>[30x]MVLGKVVGTVVASRKEPRIEGLSLLLVRACDPDGTPTGGAVVCADAVGAGVGEVVLYASGSSARQTEVTNNRPVDATIMAIVDLVEMGGDVRFRKD;>[180x]MADALGMIEVRGFVGMVEAA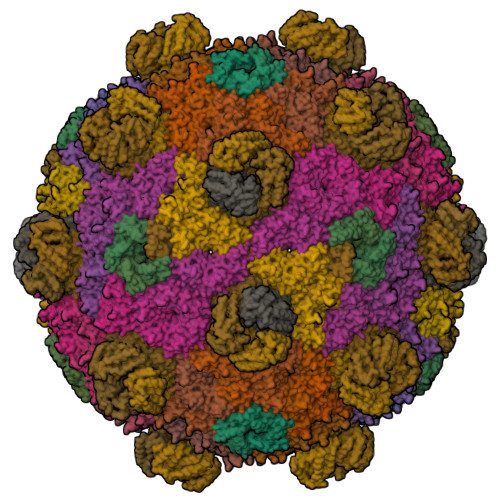DAMVKAAKVELIGYEKTGGGYVTAVVRGDVAAVKAATEAGQRAAERVGEVVAVHVIPRPHVNVDAALPLGRTPGMDKSA;>[60x]MSITLRTYIFLDALQPQLATFIGKTARGFLPVPGQASLWVEIAPGIAINRVTDAALKATKVQPAVQVVERAYGLLEVHHFDQGEVLAAGSTILDKLEVREEGRLKPQVMTHQIIRAVEAYQTQIINRNSQGMMILPGESLFILETQPAGYAVLAANEAEKAANVHLVNVTPYGAFGRLYLAGSEAEIDAAAEAAEAAIRSVSGVAQESFRDR>[4x]VSPNYDKWEMERTDITMKHKLGGGQYGEVYEGVWKKYSLTVAVKTLKEDTMEVEEFLKEAAVMKEIKHPNLVQLLGVCTREPPFYIITEFMTYGNLLDYLRECNRQEVNAVVLLYMATQISSAMEYLEKKNFIHRDLAARNCL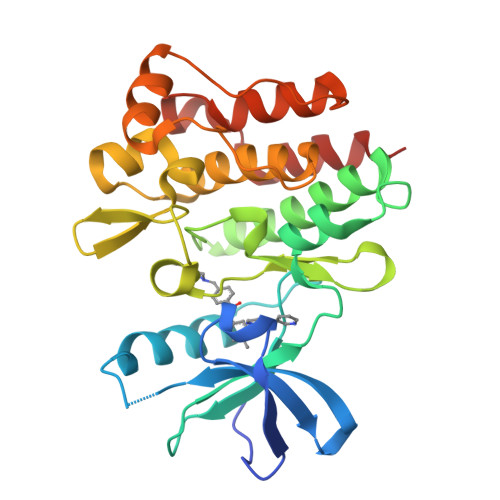VGENHLVKVADFGLSRLMTGDTYTAHAGAKFPIKWTAPESLAYNKFSIKSDVWAFGVLLWEIATYGMSPYPGIDLSQVYELLEKDYRMERPEGCPEKVYELMRACWQWNPSDRPSFAEIHQAFETMFQES3-benzyl-4-methyl-2-oxo-2H-1-benzopyran-7-yl methanesulfonate | C18 H16 O5 S | 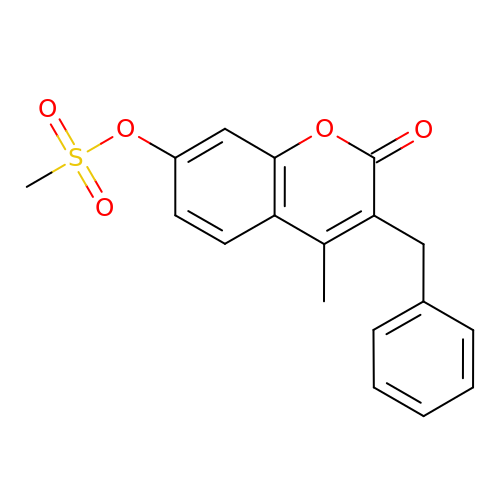FNVRQJZWEFVUOH-UHFFFAOYSA-N> MEPPTVALTVPAAALLPDGALGESIVRGRRYLSDTPAQLPDFVGNGLACRHCHPGRDGEVGTEANAAPFVGVVGRFPQYSARHGRLITLEQRIGDCFERSLNGRALALDHPALIDMLAYMSWLSQGVPVGAVVAGHGIPTLTLEREPDGVHGEALYQARCLACHGADGSGTLDADGRYLFPPLWGPRSFNTGAGMNRQATAAGFIKHGMPLGADDSLSD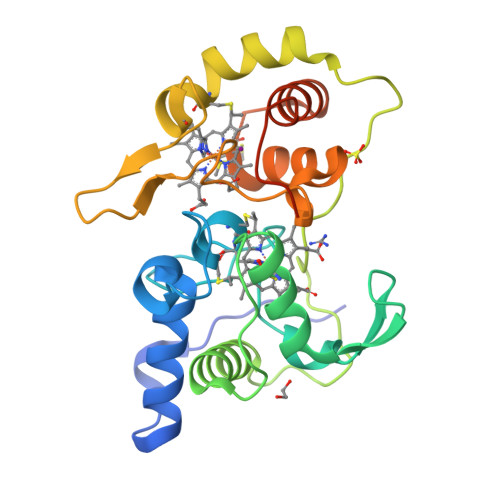EEAWDVAGFVLTHPRPLFQEPTGDAWSHPQFEK> SMEEKLENEPDFQYIPEKAPLDSVHQDDHSLRESMIQLAEGLITGTVLTQFDQLYRKKPGMTMSCAKLPQNISKNRYRDISPYDATRVILKGNEDYINANYINMEIPSSSIINQYIACQGP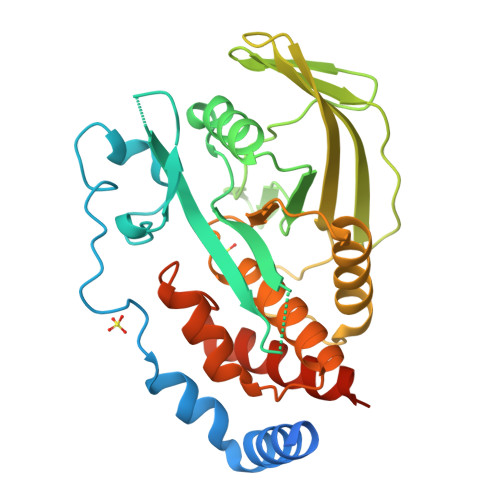LPHTCTDFWQMTWEQGSSMVVMLTTQVERGRVKCHQYWPEPTGSSSYGCYQVTCHSEEGNTAYIFRKMTLFNQEKNESRPLTQIQYIAWPDHGVPDDSSDFLDFVCHVRNKRAGKEEPVVVHCSAGIGRTGVLITMETAMCLIECNQPVYPLDIVRTMRDQRAMMIQTPSQYRFVCEAILKVYEEGFVKPLTTSTNKLT5-[3,5-dimethoxy-4-[(3-oxidanylazetidin-1-yl)methyl]phenyl]-1,3-dimethyl-pyridin-2-one | 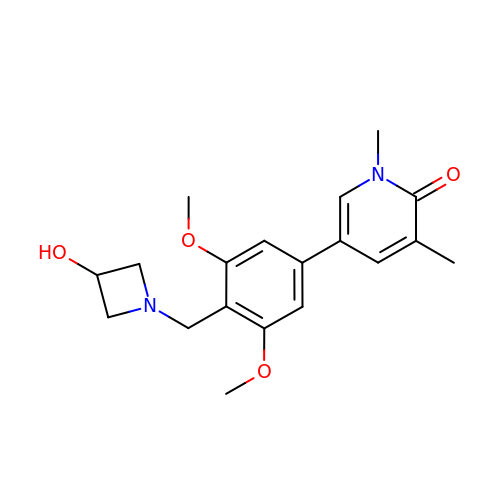C19 H24 N2 O4 | YZIWDEXMYWHXDR-UHFFFAOYSA-N> MSCPEQIVQLMHMHLDGDILPKDEHVLNEHLETCEKCRKHFYEMEKSIALV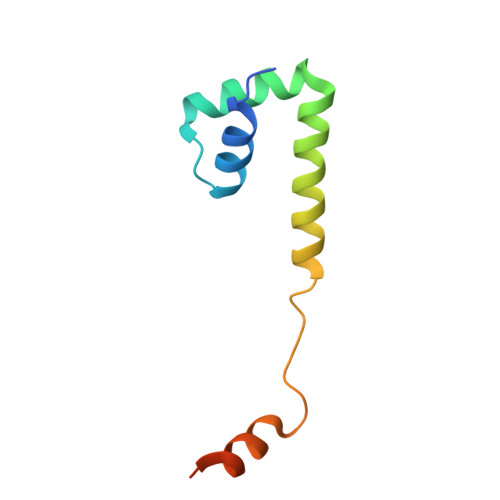RSTSHVEAPADFTANVMAKLPKEKKRASV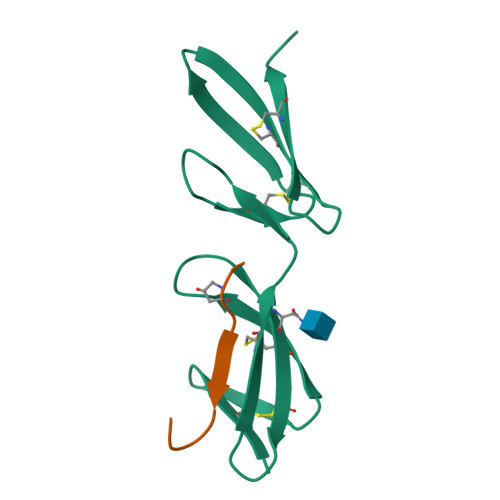>[2x]DQCIVDDITYNVQDTFHKKHEEGHMLNCTCFGQGRGRWKCDPVDQCQDSETGTFYQIGDSWEKYVHGVRYQCYCYGRGIGEWHCQPLQTYPSS;>GLPGTAGLPGMKGHRGFSGLDGY[2x]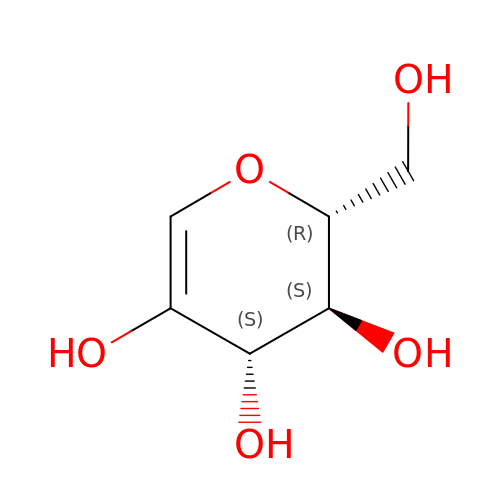1,5-anhydro-D-arabino-hex-1-enitol | C6 H10 O5 | CXKKSSKKIOZUNR-HSUXUTPPSA-N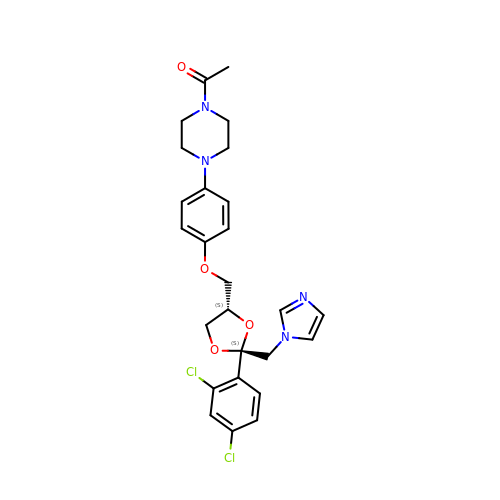CIS-1-ACETYL-4-(4-((2-(2,4-DICHLOROPHENYL)-2-(1H-IMIDAZOL-1-YLMETHYL)-1,3-DIOXOLAN-4-YL)METHOXY)PHENYL)PIPERAZINE | C26 H28 Cl2 N4 O4 | XMAYWYJOQHXEEK-JYFHCDHNSA-N ADENOSINE-5'-(DITHIO)PHOSPHATE | C10 H14 N5 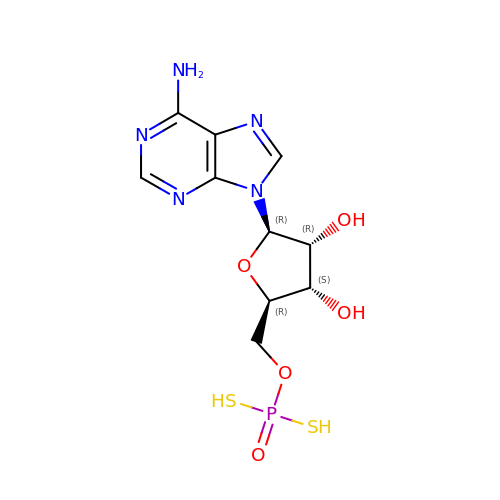O5 P S2 | RPDDEEQJNPPYRG-CPTYKQRNSA-N> MGNVREEGINMYLTDNYTPKMNQIISVTDNFRRATVAVSLSTNVMASSIKNSIGSASNRVNSLNSSLRKVQTTASSVSSTMTKLSSSINAVSGVIGSLNGSIMRLAITIAMIIDYFNKLIQKKNEFNSNIMIILIFKAKSDEVEKTKNKLLGNLKKIGGKIWNIVIKAKDMTKRVISSILGKLKQVEKRPYQGSINLKDMVSSAMGRILPKLMLFKNTFWSGVIAIKDMASGIISKVFPKLRLFAGKVWSGAIAVKDMASGILGSIKGKISDLTNGATIGVAVKKGVDLLGQEQNQKVVLESVMKRNTGKVNQIDVDDYYGSLVRMANDTPFDPEDVVAMGTKAKMISNITGGKKEKDITQAMVDVRALNMNTSSEQDVSAAFLSAAKGNMESLNTLVGENYKTFDEALEGISVKQMGLAKEMSNTIPGIISGAQTSINNGLKSIVKPFDDILGQGLKKIKTFIESGLGNLAGLSEKMAGKIGNVMNGKIIIGNKYDQMQSRSVKNGKEFSDSTQYRISNEAEKRKMMVENKQERFENHAATMIGNAPKAIVNAGSTLLQNIDFTALIDSLLPVVNLVNNLLDSINNKSPIAQGLISIFGTIVTTAFQLIGPVVEAVSPIITRIFTFLGEYAPQINNFIETLGVIWKTVWETLGPLLETGWKIIEPILGAFFNILDKVCKIVKDICKWWQTMINKIKNGSITGTVLNLVEKSKKNYKDNPYAGTKAGDSGKAYSGKKGNNAFGLNYVPYNDYQTRLHEGEMVLTKQEANQ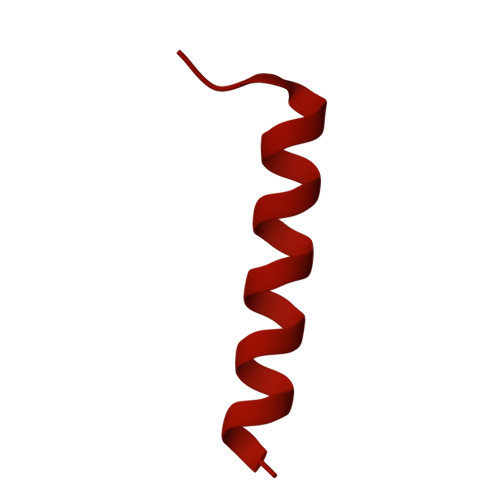YRSRKNGGNINIAKLADTIVIREEADIEKITSKLVASIQLAQLGGVL3-[5-(2-cyclohexylethyl)-4-ethyl-1,2,4-triazol-3-yl]-N-naphthalen-1-yl-propanamide 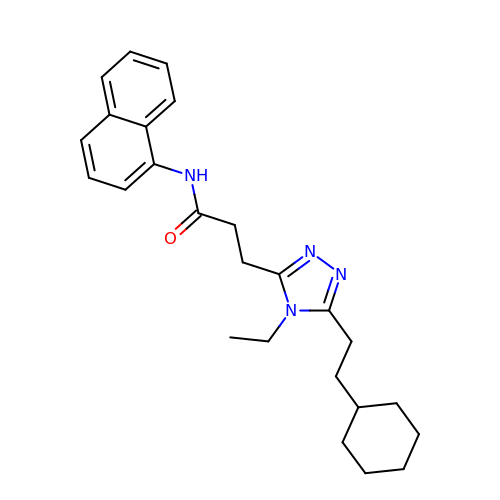| C25 H32 N4 O | SZWIGRNIVUKPOZ-UHFFFAOYSA-N> GSHMPINLLGKTLWLGLISFAVLGTVNAAQYNAVVSTTPQGDEFSSINAALKSAPKDDTPFIIFLKNGVYTERLEVARSHVTLKGENRDGTVIGANTAAGMLNPQGEKWGTSGSSTVLVNAPNFTAENLTIRNDFDFPANKKKADTDPTKLKDTQAVALLLAENSDKARFKAVKLEGYQDTLYSKTGSRSYFSDCEISGHVDFIFGSGITVFDNCNIVARDRSDIEPPYGYITAPSTLTTSPYGLIFINSRLTKEPGVPANSFALGR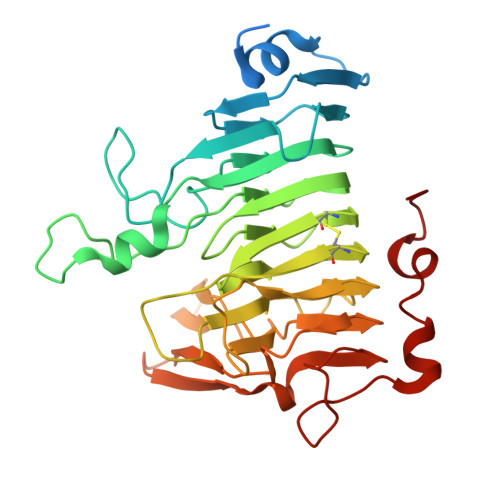PWHPTTTFADGRYADPAAIGQSVFINTTMDDHIYGWDKMSGKDKQGEKIWFYPQDSRFFEANSQGPGAAINEGRRQLSAEQLKAFTLPMIFPDWAVH> LSDKKAS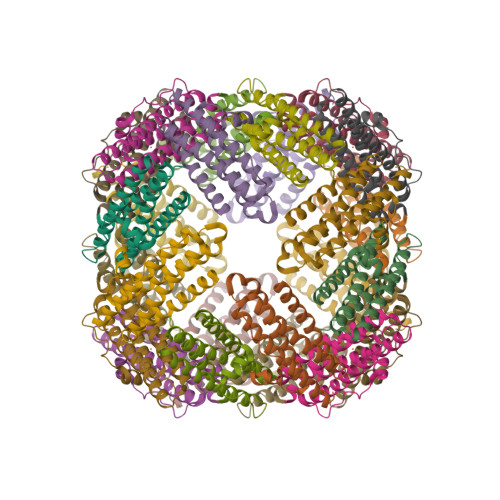DVADLLQKQLSTYNDLHLTLKHVHWNVVGPNEIGVHEMIDPQVELVRGYADEVAERIATLGKSPKGTPGAIIKDRTWDDYSVERDTVQAHLAALDLVYNGVIEDTRKSIEKLEDLDLVSQDLLIAHAGELEKFQWFVRAHLE> MSEIGTGFPFDPHYVEVLGERMHYVDVGPRDGTPVLFLHGNPTSSYLWRNIIPHVAPSHRCIAPDLIGMGKSDKPDLDYFFDD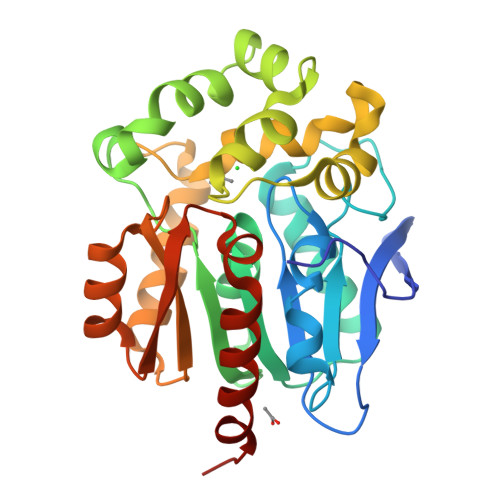HVRYLDAFIEALGLEEVVLVIHDWGSALGFHWAKRNPERVKGIACMEFIRPFPTWDEWPEFARETFQAFRTADVGRELIIDQNAFIEGALPKCVVRPLTEVEMDHYREPFLKPVDREPLWRFPNELPIAGEPANIVALVEAYMNWLHQSPVPKLLFWGTPGVLIPPAEAARLAESLPNCKTVDIGPGLHYLQEDNPDLIGSEIARWLPALHHHHHH> MEHRYNVFNDTPRGNHWMGSSVSGSPRPSYSSRPNVNTTRRFQYSDDEPAEKIRPLRSRSFKSTESNISDEKSRISERDSKDRYINGDKKVDIYSLPLISTDVLEISKQRTFAVILFLIIQCYKIYDLVILKSGLPLSGLLFKNYRFNFISKYFIIDSFFLYVLPSFNIPRLTFKPWVVYLQILAMLLLNIFISSDHEFVLISLIMTTWRKLYTKELSVTGSAINHHRIFDSSAHFKGALTIKILPENTAMFNPLHESYCLPMDTNLFKINSIDVPIRINSTEEIEYIELEYRDLYTNSVELRSLSKKDFKIIDNPKSFLKKDQSVLKSHSNDFEEGSTIRYLAVTLQDIGFYQIKKIVDSKKLNLKIHQSHLVVPYCPIASITGTGSNDRCIGDSDNVSFEIQGVPPMKLAYSKIVNGQTFSYVDSSLQPEYFESPLQSSKSKQSFTQGELNDLKWGRNQPVNINLDSSITQDGKFAYKIDKITDGLGNVVDFTSLPEELKKRYDLSYNFNVHEVPRAALEERFDPKSPTKRSIAIVFEEIKNWISDIPYVISLSYTDAQDKSKKIMNVTTDSLTKVLQADLPGSYNLEYIESKFCPGEIVGKSNVLVTMPVAPTMEVKSFPILDQCVGQVGLNFELSFTGAPPYYYNTKIYKLENGERKLYDAKRYTSEGTRNRFSYSPPKEGNYEIVFDTVSNKLFTEPIKLEPVKEYTFKTSMRVKPSASLKLHHDLKLCLGDHSSVPVALKGQGPFTLTYDIIETFSSKRKTFEIKEIKTNEYVIKTPVFTTGGDYILSLVSIKDSTGCVVGLSQPDAKIQVRRDIPSAAFNFFEPIKEAKIKHGSVTEIPLKLSGE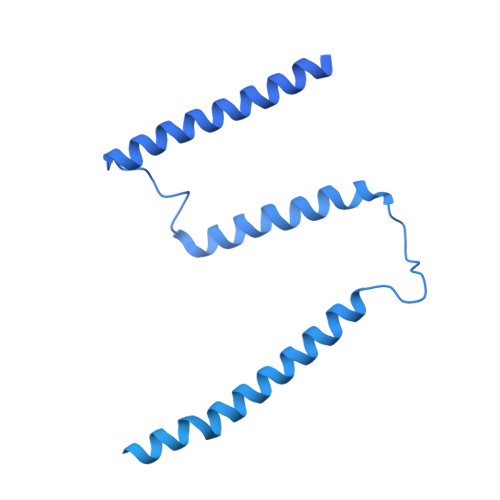GPFTVKFKHMDYDGNIVKEFENKFQNSYKPALKVSKEGLYQLVDIRDSSCQGNVIYRNSLYKVSFLEKPKFAIQDNHHITKVTENLFSKEEVCQGMEGTVDLALFGSPPFILEYDLMAPNGHISTKKIQVATKYASLKLPNQIPGEYITTIKAIFDGNYGESDIHFREHQSELIIKQTVHPIPDVAFADGGKTLRACAANVDQISFLEPINLKFLQGESPFSITFSVYHESTSRTDQYTIDNIDSENFSFEKLYEGMKLGNHAITIDSVVDANGCVNSLISGPRNQILVSITDAPKIHILDPSTEYCVGDYVAYQLNGVAPFMIKYEFNGIPLKSKERSSQFVRLASEPGIISITSLQDSSSQCIVDFTNPKLKSEFDDLSLNIHPIPSVTVSQGNYVTEDIREGDQAEVIFSFEGTPPFSLTYVRTEETDGKHGKRRSQVVETHKVTDIYSHEYKVITSLQGTYEAIEITDAYCFAKNDLFFNN2-isoquinolin-2-ium-2-yl-1-phenyl-ethanone 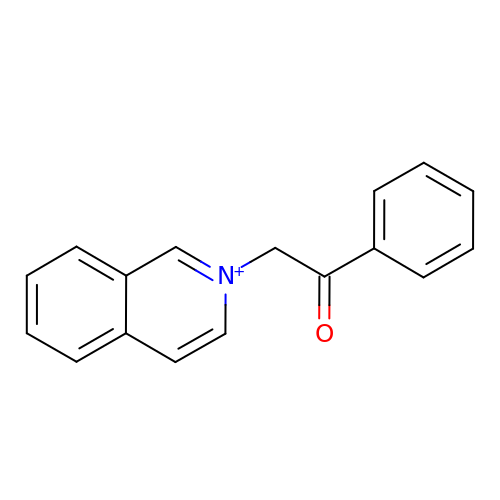| C17 H14 N O | LIAJGECMVWAMNA-UHFFFAOYSA-N>MGEVFKEVKEKFERYKFDVVYVDREYPVSSNNLNVFFEIGERNSFSGLLINEGQAVIDVLLLKKSHEGLSPIPGEGTGIQLSAGQILKFYNVPIAEIIVEYDPSNVSGVSSNVKLKGTIHPLFEVPSQISIENFQPTENYLIYSGFGTSLPQTYTIPANGYLIISITNTSTGNIGQITLTIGSTTMTFNLQTG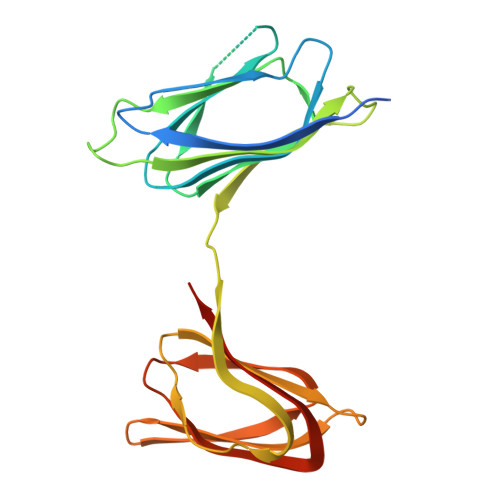ENKIPVIAGTQITNMTLTSSSAILIYEEVIHHHHHH[2x]>[2x]GAMGKCPTKVVLLRNM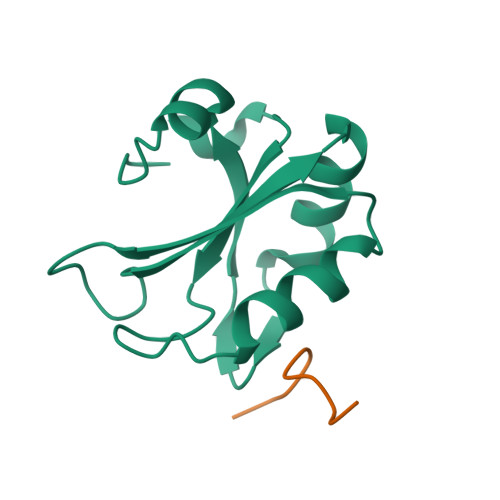VGAGEVDEDLEVETKEECEKYGKVGKCVIFEIPGAPDDEAVRIFLEFERVESAIKAVVDLNGRYFGGRVVKACFYNLDKFRVLDLAEQV;>KRKSRWDETP[2x]> GSHMPEEEKAARLFIEALEKGDPELMRKVISPDTRMEDNGREFTGDEVVEYVKEIQKRGEQWHLRRYTKEGNSWRFEVQVDNNGQTEQWEVQIEV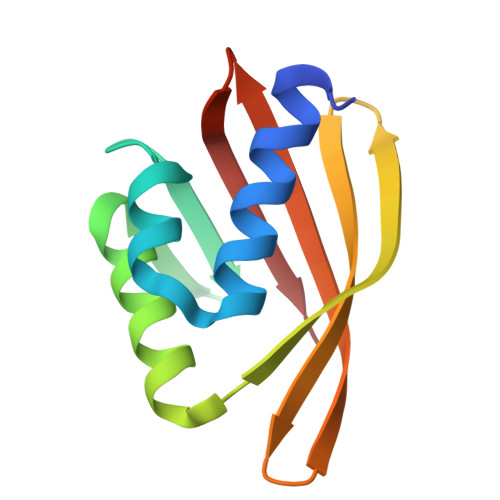RNGRIKRVTITHV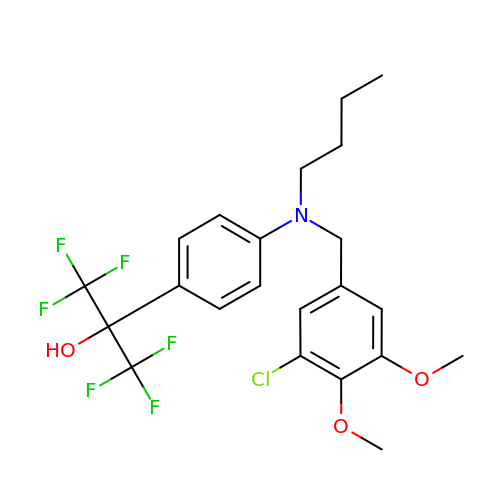2-{4-[butyl(3-chloro-4,5-dimethoxybenzyl)amino]phenyl}-1,1,1,3,3,3-hexafluoropropan-2-ol | C22 H24 Cl F6 N O3 | QKFWYOZIIUVZRC-UHFFFAOYSA-N>CGTACG[2x]

Variolin B (9-amino-5-(2-aminopyrimidin-4-yl)-1H-pyrido[3,4]pyrrolo[3,5-c]pyrimidin-4-one) is a natural anti-tumour and antiviral compound. However, experimental evidence of variolin B acting as a cyclin-dependent kinase inhibitor (both on CDK1 and CDK2) moved the attention to its interaction with these essential proteins. Nevertheless, here we report the high-resolution structure of a complex showing that variolin B also can bind to a multi-stranded DNA in an intercalative fashion. Our structure confirms that variolin B is indeed a DNA intercalator.

In the final model for the DNA-variolin B complex the DNA adopts a B-form conformation only along the four central base pairs of the d(CGTACG)2 duplex. As in previously reported isomorphous structures including Co2+ ions, the strands at both ends of the DNA duplex are distorted and interact with symmetry-related DNA molecules. At the other end, cytosine C7 is rotated so that it pairs the guanine G6 of a symmetry-related duplex, forming a pseudo-Holliday junction that involves four DNA duplexes. Such association generates an intercalation site between the interduplex G6 · C7 and the intraduplex C5 · G8 base pairs. While this particular crystal packing is caused mainly by DNA-DNA and DNA-ion interactions, a DNA intercalator is the keystone required to fix the whole structure. The electron density for the intercalator is strong but does not allow to define a single orientation of the compound. Instead, the final model shows two drug molecules in different orientations, each with half occupancy. One of the orientations enables a bifurcated hydrogen bond between the −NH2 group of the tricyclic moiety of the drug and the guanine G6 phosphate. Once intercalated, variolin B adopts a quasi-planar conformation. The 2-aminopyrimidine ring is only 10.5° out of the pyridopyrrolopyrimidine mean plane in one drug molecule, whereas in the other this angle is 8.4°.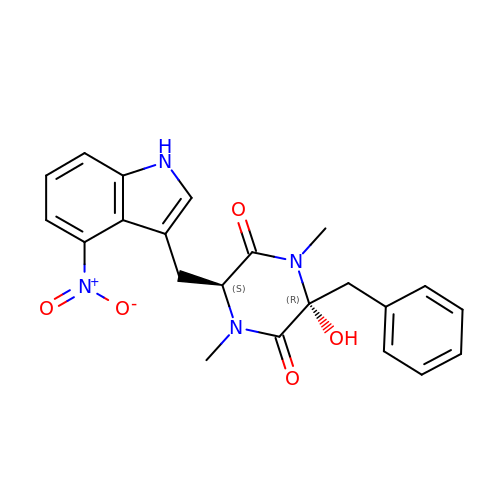(3~{R},6~{S})-1,4-dimethyl-6-[(4-nitro-1~{H}-indol-3-yl)methyl]-3-oxidanyl-3-(phenylmethyl)piperazine-2,5-dione | C22 H22 N4 O5 | PCCPGPMTZJOQFC-PGRDOPGGSA-N>[4x]MKKYNVCIVGGGSTYTPGFLKSFVRLQNEFPMEKLVLFDIDAERQQPIGEFGKILFSERFPELDFSYTTDPAEAYKDMDFIFMQMRAGGLPMRREDEHISLHLGRIGQETCGAGGMAYGLRSCVDMIESIHQIRQYSPNAWILNYSNPAAIVAEALRREFPDDNRILNICDQPENIMRSVSRLLNVSWEDLDPVYFGLNHYGWFTHVYDRK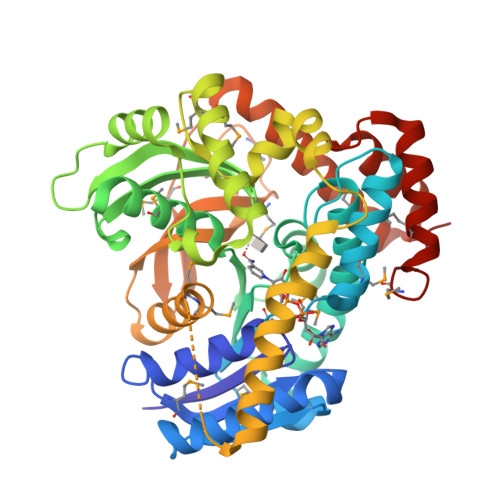TGEDLLPEIKKIIKEKGFLPQDAEQRDQSWLDTYGFVQTMMEDFPDFLPNTYDGYYLYPDYKFSHLNPDYTRADEVIDGREKRVFAECREVIARGELGDRFDTISDAHAEMMIKVAEAIAYNKNTRFIVIVKNEGAIANMQDDAMVELVCELGINGPRRMAVGNIPQFYLGLLVQQVSSEKLLVDAYYEHSYQKALEAFTLNRLINDAKKAREILDAMIEVNKGMWPELK>ATAAEIAALPRQKVELVDPPFVHAHSQVAEGGPKVVEFTMV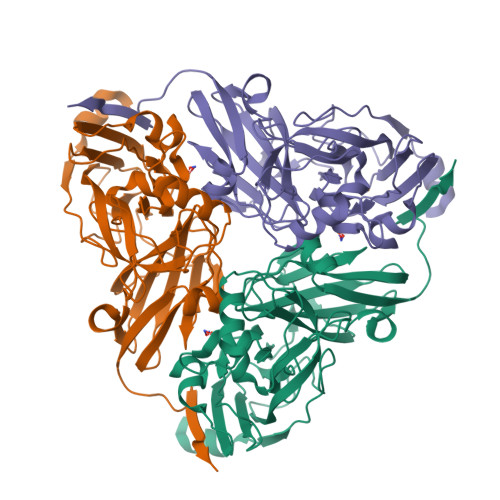IEEKKIVIDDAGTEVHAMAFNGTVPGPLMVVHQDDYLELTLINPETNTLMHNIDFHAATGALGGGGLTEINPGEKTILRFKATKPGVFVYHCAPPGMVPWHVVSGMNGAIMVLPREGLHDGKGKALTYDKIYYVGEQDFYVPRDENGKYKKYEAPGDAYEDTVKVMRTLTPTHVVFNGAVGALTGDKAMTAAVGEKVLIVHSQANRDTRPHLLGGHGDYVWATGKFNTPPDVDQETWFIPGGAAGAAFYTFQQPGIYAYVNHNLIEAFELGAAAHFKVTGEWNDDLMTSVLAPSGTIEGR[3x]>[2x]MELWLVRHGETLWNREGRL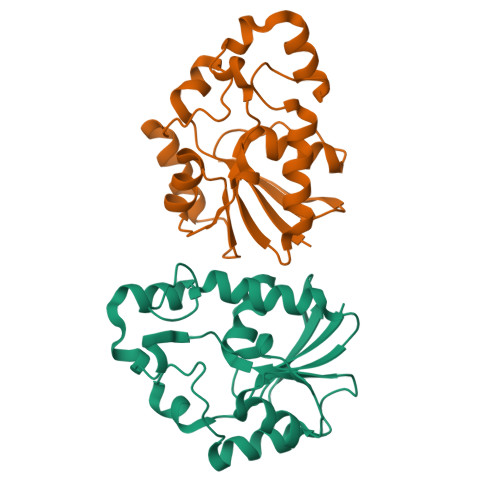LGWTDLPLTAEGEAQARRLKGALPSLPAFSSDLLRARRTAELAGFSPRLYPELREIHFGALEGALHETLDPRYKEALLRFQGFHPPGGESLSAFQERVFRFLEGLKAPAVLFTHGGVVRAVLRALGEDGLVPPGSAVAVDWPRRVLVRLALDGEEATG> MSLNMFWFLPTHGDGHYLGTEEGSRPVDHGYLQQIAQAADRLGYTGVLIPTGRSCEDAWLVAASMIPVTQRLKFLVALRPSVTSPTVAARQAATLDRLSNGRALFNLVTGSDPQELAGDGVFLDHSERYEASAEFTQVWRRLLQRETVDFNGKHIHVRGAKLLFPAIQQPYPPLYFGGSSDVAQELAAEQVDLYLTWGEPPELVKEKIEQVRAKAAAHGRKIRFGIRLHVIVRETNDEAWQAAERLISHLDDETIAKAQAAFA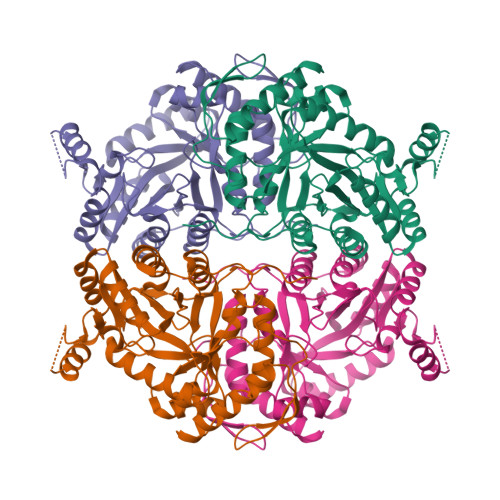RTDSVGQQRMAALHNGKRDNLEISPNLWAGVGLVRGGAGTALVGDGPTVAARINEYAALGIDSFVLSGYPHLEEAYRVGELLFPLLDVAIPEIPQPQPLNPQGEAVANDFIPRKVAQS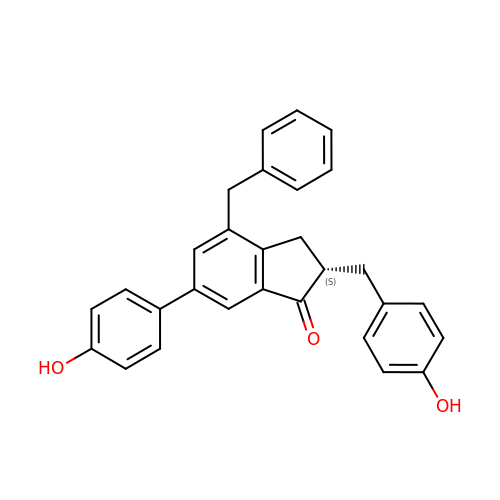(2~{S})-6-(4-hydroxyphenyl)-2-[(4-hydroxyphenyl)methyl]-4-(phenylmethyl)-2,3-dihydroinden-1-one | C29 H24 O3 | BBBVODRPSLPZKR-DEOSSOPVSA-N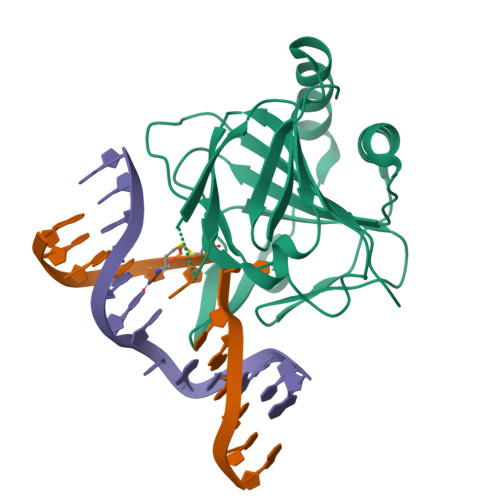>[2x]SHSWRHIRAEGLDSSYTVLFGKAEADEIFQELEKEVEYFTGALARVQVFGKWHSVPRKQATYGDAGLTYTFSGLTLSPKPWIPVLERIRDHVSGVTGQTFNFVLINRYKDGSDHICEHRDDERELAPGSPIASVSFGASRDFVFRHKDSRGKSPSRRVAVVRLPLAHGSLLMMNHPTNTHWYHSLPVRKKVLAPRVNLTFRKILLTKK> MNPIHDRTSDYHKYLKVKQGDSDLFKLTVSDKRYIWYNPDPKERDSYECGEIVSETSDSFTFKTVDGQDRQVKKDDANQRNPIKFDGVEDMSELSYLNEPAVFHNLRVRYNQDLIYTYSGLFLVAVNPFKRIPIYTQEMVDIFKGRRRNEVAPHIFAISDVAYRSMLDDRQNQSLLITGESGAGKTENTKKVIQYLASVAGRNQANGSGVLEQQILQANPILEAFGNAKTTRNNNSSRFGKFIEIQFNNAGFISGASIQSYLLEKSRVVFQSETERNYHIFYQLLAGATAEEKKALHLAGPESFNYLNQSGCV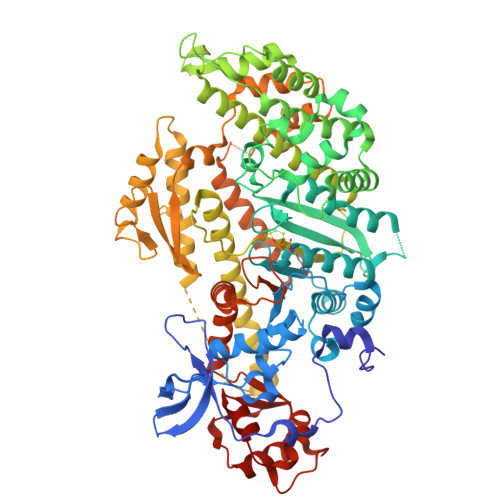DIKGVSDSEEFKITRQAMDIVGFSQEEQMSIFKIIAGILHLGNIKFEKGAGEGAVLKDKTALNAASTVFGVNPSVLEKALMEPRILAGRDLVAQHLNVEKSSSSRDALVKALYGRLFLWLVKKINNVLCQERKAYFIGVLDISGFEIFKVNSFEQLCINYTNEKLQQFFNHHMFKLEQEEYLKEKINWTFIDFGLDSQATIDLIDGRQPPGILALLDEQSVFPNATDNTLITKLHSHFSKKNAKYEEPRFSKTEFGVTHYAGQVMYEIQDWLEKNKDPLQQDLELCFKDSSDNVVTKLFNDPNIASRAKKGANFITVAAQYKEQLASLMATLETTNPHFVRCIIPNNKQLPAKLEDKVVLDQLRCNGVLEGIRITRKGFPNRIIYADFVKRYYLLAPNVPRDAEDSQKATDAVLKHLNIDPEQYRFGITKIFFRAGQLARIEEAREPN> RADVKPVTVKLVDSQATMETRSLFAFMQEQRRHSIMFGHQHETTQGLTITRTDGTQSDTFNAVGDFAAVYGWDTLSIVAPKAEGDIVAQVKKAYARGGIITVSSHFDNPKTDTQKGVWPVGTSWDQTP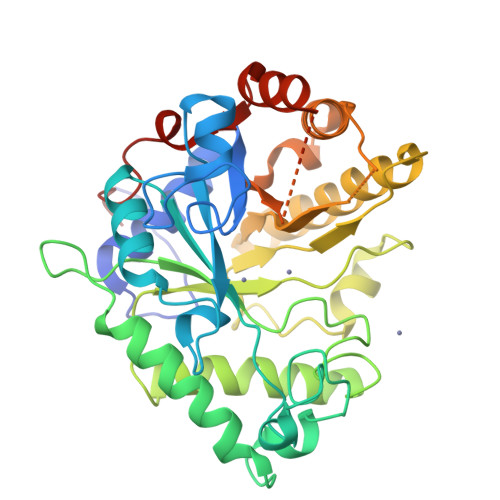AVVDSLPGGAYNPVLNGYLDQVAEWANNLKDEQGRLIPVIFRLYHENTGSWFWWGDKQSTPEQYKQLFRYSVEYLRDVKGVRNFLYAYSPNNFWDVTEANYLERYPGDEWVDVLGFDTYGPVADNADWFRNVVANAALVARMAEARGKIPVISEIGIRAPDIEAGLYDNQWYRKLISGLKADPDAREIAFLLVWRNAPQGVPGPNGTQVPHYWVPANRPENINNGTLEDFQAFYADEFTAFNRDIEQVYQRPTLIVK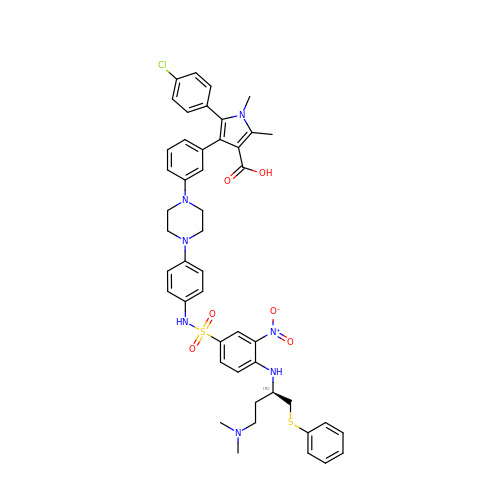5-(4-chlorophenyl)-4-{3-[4-(4-{[(4-{[(2R)-4-(dimethylamino)-1-(phenylsulfanyl)butan-2-yl]amino}-3-nitrophenyl)sulfonyl]amino}phenyl)piperazin-1-yl]phenyl}-1,2-dimethyl-1H-pyrrole-3-carboxylic acid | C47 H50 Cl N7 O6 S2 | IUXZRSUDCUOHPK-DIPNUNPCSA-N>[2x]EENFSRSYPCDEKKQNDSVIAECSNRRLQEVPQTVGKYVTELDLSDNFITHITNESFQGLQNLTKINLNHNPNVQHQNGNPGIQSNGLNITDGAFLNLKNLRELLLEDNQLPQIPSGLPESLTELSLIQNNIYNITKEGISRLINLKNLYLAWNCYFNKVCEKTNIEDGVFETLTNLELLSLSFNSLSHVPPKLPSSLRKLFLSNTQIKYISEEDFKGLINLTLLDLSGNCPRCFNAPFPCVPCDGGASINIDRFAFQNLTQLRYLNLSSTSLRKINAAWFKNMPHLKVLDLEFNYLVGEIASGAFLTMLPRLEILDLSFNYIKGSYPQHINISRNFSKLLSLRALHLRGYVFQELREDDFQPLMQLPNLSTINLGINFIKQIDFKLFQNFSNLEIIYLSENRISPLVKDTRQSYANSSSFQRHIRKRRSTDFEFDP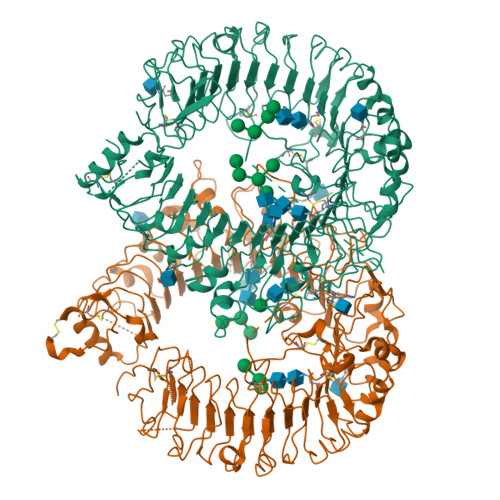HSNFYHFTRPLIKPQCAAYGKALDLSLNSIFFIGPNQFENLPDIACLNLSANSNAQVLSGTEFSAIPHVKYLDLTNNRLDFDNASALTELSDLEVLDLSYNSHYFRIAGVTHHLEFIQNFTNLKVLNLSHNNIYTLTDKYNLESKSLVELVFSGNRLDILWNDDDNRYISIFKGLKNLTRLDLSLNRLKHIPNEAFLNLPASLTELHINDNMLKFFNWTLLQQFPRLELLDLRGNKLLFLTDSLSDFTSSLRTLLLSHNRISHLPSGFLSEVSSLKHLDLSSNLLKTINKSALETKTTTKLSMLELHGNPFECTCDIGDFRRWMDEHLNVKIPRLVDVICASPGDQRGKSIVSLELTTCVSDVT>PVVIKTEGPAWTPLEPKLITRLADTVRTKGLRSPITMAEVEALMSSPLLPHDVTNLMRVILGPAPY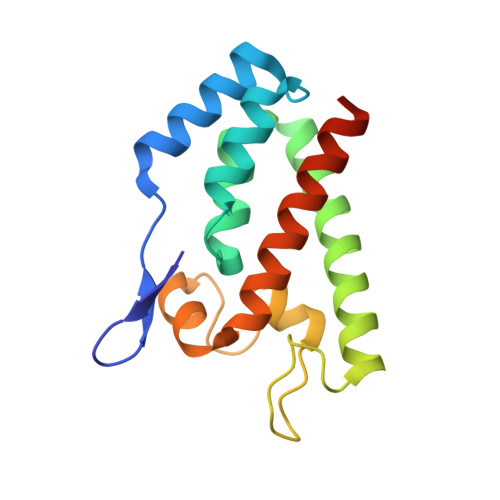ALWMDAWGVQLQTVIAAATRDPRHPANGQGRGERTNLNRLKGLADGMVGNPQGQAALLRPGELVAITASALQAFREVARLAEPAGPWA[2x]>MPFTIDSARGIFPNTLAADVVPATIARFSQLNAEDQLALIWFAYLEMGKTLTIAAPGAASMQLAENALKEIQAMGPLQQTQAMCDLANRADTPLCRTYASWSPNIKLGFWYRLGELMEQGFVAPIPAGYQLSANANAVLATIQGLESGQQITVLRNAVVDMGFTAGKDGKRIAEPVVPPQDTASRTKVSIEGVTNATVLNYMDNLNANDFDTLIELFTSDGALQPPFQRPIVGKENVLRFFREECQNLKLIPERGVTEPAED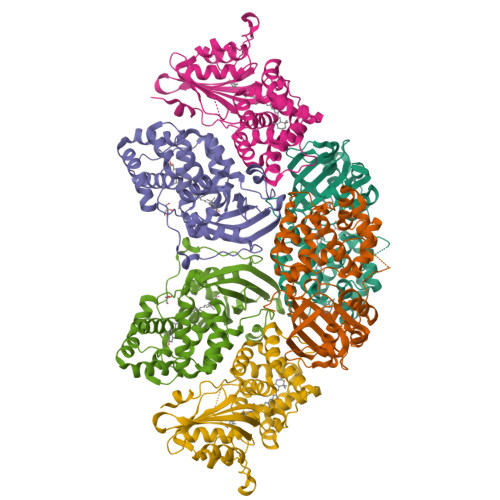GFTQIKVTGKVQTPWFGGNVGMNIAWRFLLNPEGKIFFVAIDLLASPKELLNFARHHHHHH[6x]>[5x]QDMVSPPPPIADEPLTVNTGIYLIECYSLDDKAETFKVNAFLSLSWKDRRLAFDPVRSGVRVKTYEPEAIWIPEIRFVNVENARDADVVDISVSPDGTVQYLERFSARVLS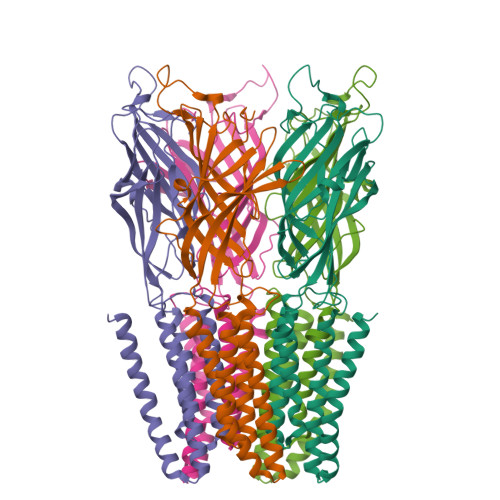PLDFRRYPFDSQTLHIYLIVRSVDTRNIVLAVDLEKVGKNDDVFLTGWDIESFTAVVKPANFALEDRLESKLDYQLRISRQYFSYIPNIILPMLFILFISWTAFWSTSYEANVTLVVSTLIAHIAFNILVETNLAKTPYMTYTGAIIFMIYLFYFVAVIEVTVQHYLKVESQPARAASITRASRIAFPVVFLLANIILAFLFFGF Proton-coupled Oligopeptide Transporters (POTs) of the Major Facilitator Superfamily (MFS) mediate the uptake of short di- and tripeptides in all phyla of life. The E. coli genome codes for four different POTs, known as Di- and tripeptide permeases A-D (DtpA-D). DtpA and B exhibit a prototypical substrate preference similar to the human PepT1 transporter, while DtpC and D have been classified as atypical POTs, because DtpC prefers dipeptides in particular those with a lysine residue in the second position. The DtpC structure revealed the expected and well-known MFS transporter fold, with twelve transmembrane helices (TMs) organized in two helical bundles and additional two TMs specific for the POT family (known as HA and HB domains).

DtpC in complex with the conformation specific nanobody 26 turned out to be more rigid and a significant fraction of the sample dimeric, allowing us to reconstruct DtpC to 2.7 Å resolution. Therefore, we performed a local refinement, focused on one copy of the membrane protein, which extended the resolution of the reconstruction to 2.7 Å and improved the accuracy of the atomic model for subsequent structural analysis. The peptide binding site of DtpC is exposed to the cytoplasmic side. In the case of the here described DtpC structure, the IF state is open. Tight closure of both bundles above the binding site is mediated by a salt bridge between D43 (TM2, N-bundle) and R294 (TM7, C-bundle) and hydrogen bonds between H37 (TM1, N-bundle) and D293 (TM7) as well as R28 (TM1) and N421 (TM11, C-bundle). In DtpC, the E1XXE2R motif, has evolved to Q1XXE2Y (where Q1 = N17, E2 = E20, Y=Y21). In DtpC, we now observe that the side chain pocket has a different architecture and characteristic in comparison with the one of canonical POTs. It displays an overall more acidic groove caused by the presence of the aspartate residue 392, conserved among atypical POTs. By replacing the phenyl group with a lysine side chain (generating the known DtpC dipeptide substrate Ala-Lys instead of Ala-Phe), we postulate a putative salt bridge between the carboxyl group of D392 and the ε-amino group of the lysine side chain. This observation, together with previous biochemical work allows us to hypothesize that the selectivity of DtpC for dipeptides with C-terminal lysine or arginine residues is caused by swapping a salt bridge between the recurrent carboxyl group of the peptide terminus and the transporter (R21Y mutation), to a side chain specific salt bridge with D392.

> MKTPSQPRAIYYIVAIQIWEYFSFYGMRALLILYLTHQLGFDDNHAISLFSAYASLVYVTPILGGWLADRLLGNRTAVIAGALLMTLGHVVLGIDTNSTFSLYLALAIIICGYGLFKSNISCLLGELYDENDHRRDGGFSLLYAAGNIGSIAAPIACGLAAQWYGWHVGFALAGGGMFIGLLIFLSGHRHFQSTRSMDKKALTSVKFALPVWSWLVVMLCLAPVFFTLLLENDWSGYLLAIVCLIAAQIIARMMIKFPEHRRALWQIVLLMFVGTLFWVLAQQGGSTISLFIDRFVNRQAFNIEVPTALFQSVNAIAVMLAGVVLAWLASPESRGNSTLRVWLKFAFGLLLMACGFMLLAFDARHAAADGQASMGVMISGLALMGFAELFIDPVAIAQITRLKMSGVLTGIYMLATGAVANWLAGVVAQQTTESQISGMAIAAYQRFFSQMGEWTLACVAIIVVLAFATRFLFSTPTNMIQESND> MPKRGKKGAVAEDGDELRTEPEAKKSKTAAKKNDKEAAGEGPALYEDPPDQKTSPSGKPATLKICSWNVDGLRAWIKKKGLDWVKEEAPDILCLQETKCSENKLPAELQELPGLSHQYWSAPSDKEG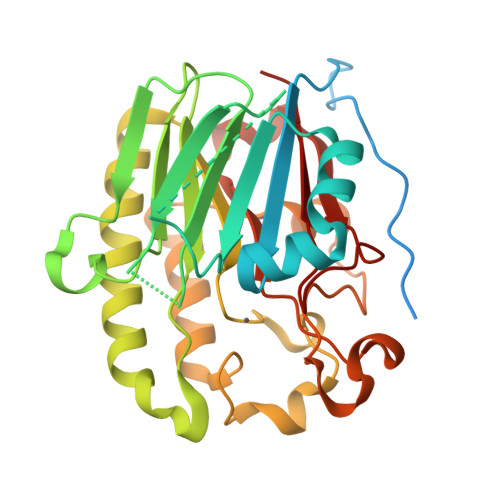YSGVGLLSRQCPLKVSYGIGDEEHDQEGRVIVAEFDSFVLVTAYVPNAGRGLVRLEYRQRWDEAFRKFLKGLASRKPLVLCGDLNVAHEEIDLRNPKGNKKNAGFTPQERQGFGELLQAVPLADSFRHLYPNTPYAYTFWTYMMNARSKNVGWRLDYFLLSHSLLPALCDSKIRSKALGSDHCPITLYLAL>[2x]MGKFGFFDDANKEYVITVPRTPYPWINYLGTENFFSLISNTAGGYSFYRDA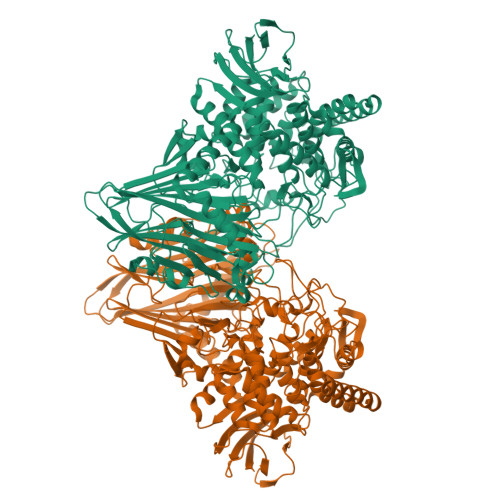RLRRITRYRYNNVPIDMGGRYFYIYDNGDFWSPGWSPVKRELESYESRHGLGYTKIAGKRNGIKAEVTFFVPLNYNGEVQKLILKNEGQDKKKITLFSFIEFSLWNAYDDMTNFQRNFSTGEVEIEGSVIYHKTEYRERRNHYAFYSVNAKISGFDSDRDSFIGLYNGFDAPQAVVNGKSNNSVADGWAPIASHSIEIELNPGEQKEYVFIIGYVENKDEEKWESKGVINKKKAYEMIEQFNTVEKVDKAFEELKSYWNALLSKYFLESHDEKLNRMVNIWNQYQSMVTFNMSRSASYFESGIGRGMGFRDSNQDLLGFVHQIPERARERLLDLAATQLEDGSAYHQYQPLTKKGNNEIGSNFNDDPLWLILATAAYIKETGDYSILKEQVPFNNDPSKADTMFEHLTRSFYHVVNNLGPHGLPLIGRADWNDSLNLNSFSTVPDESFQTTTSKDGKVAESVMIAGMFVFIGKDYVKLSEYMGLEEEARKAQQHIDAMKEAILKYGYDGEWFLRAYDDFGRKVGSKENEEGKIFIESQGFSVMAEIGLEDGKALKALDSVKKYLDTPYGLVLQNPAFTRYYIEYGEISTYPPGYKENAGIFSHNNAWIISAETVVGRGDMAFDYYRKIAPAYIEDVSDIHKLEPYVYAQMVAGKDAKRHGEAKNSWLTGTAAWNFVAISQWILGVKPDYDGLKIDPSIPKAWDGYKVTRYFRGSTYEITVKNPNHVSKGVAKITVDGNEISGNILPVFNDGKTHKVEVIMGLEHHHHHH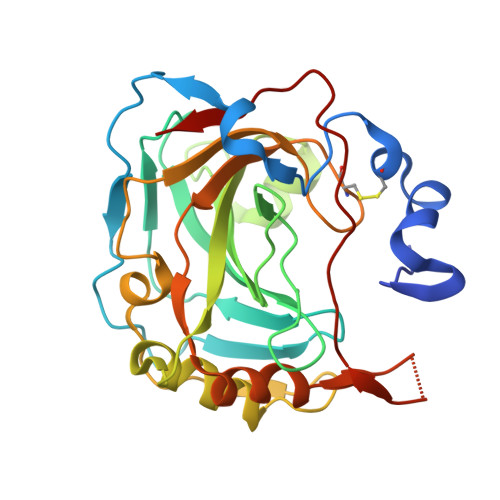>GPGSGDPYWAYSGAYGPEHWVTSSVSCGGSHQSPIDILDHHARVGDEYQELQLDGFDNESSNKTWMKNTGKTVAILLKDDYFVSGAGLPGRFKAEKVEFHWGHSNGSAGSEHSVNGRRFPVEMQIFFYNPDDFDSFQTAISENRIIGAMAIFFQVSPRDNSALDPIIHGLKGVVHHEKETFLDPFILRDLLPASLGSYYRYTGSLTTPPCSEIVEWIVFRRPVPISYHQLEAFYSIFTTEQQDHVKSVEYLRNNFRPQQALNDRVVSKS[4x]> GGIQMPVFHTRTIESILEPVAQQISHLVIMHEEGEVDGKAIPDLTAPVSAVQAAVSNLVRVGKETVQTTEDQILKRDMPPAFIKVENACTK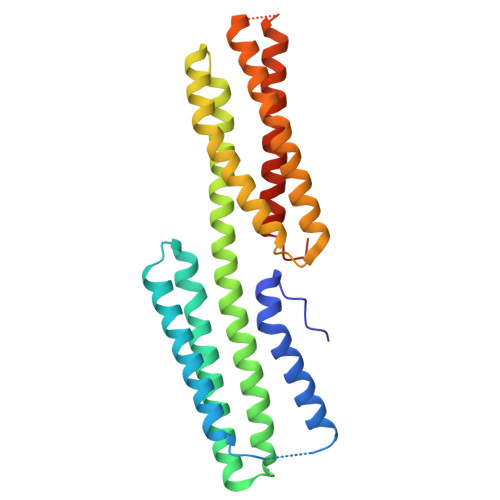LVRAAQMLQADPYSVPARDYLIDGSRGILSGTSDLLLTFDEAEVRKIIRVCKGILEYLTVAEVVETMEDLVTYTKNLGPGMTKMAKMIDERQQELTHQEHRVMLVNSMNTVKELLPVLISAMKIFVTTKNTKSQGIEEALKNRNFTVEKMSAEINEIIRVLQLTSWDEDAWA> MERTPVEENGRLQVVGTALLNQHNKPFQLRGISTHGLQWFGQFANKDAFQTLRDDWKANVVRLAMYTDPNANGYIAQPEWLKAKVKEGVQAALDLGMYVIIDWHILNDNDPNLYKEQAKRFFAEMAREYGKYPNVIYEIANEPNGNDVTWEEKIRPYADEVIRTIRSIDRDNLIIVGTGTWSQDVDDVASDPLPYKNIMYAVHFYSGTHTQWLRDRVDAALQAGTPVFVSEWGTSDASGDGGPYLEEAEKWIEFLNERGISWVNWSLCDKNEASAALRPGADPHGGWGDDHL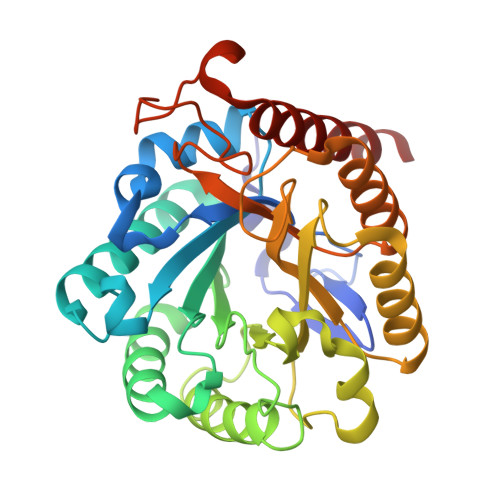SDSGRFIKAKLIEALEHHHHHH>[2x]MERDGTFNL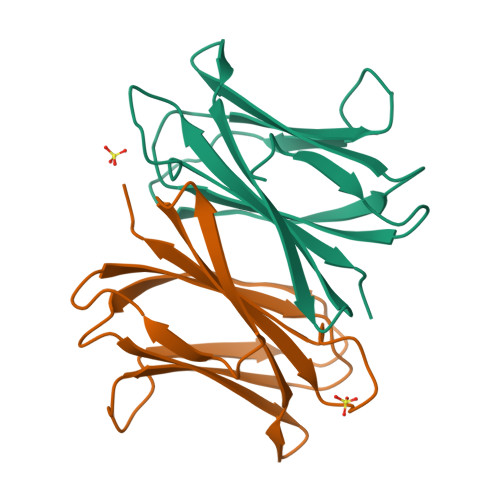PPHIKFGVTALTHAANDQTIDIYIDDDPKPAATFKGAGAQDQNLGTKVLDSGNGRVRVIVMANGRPSRLGSRQVDIFKKSYFGIIGSEDGADDDYNDGIVFLNWPLG> IVGGYTCQENSVPYQVSLNSGYHFCGGSLINDQWVVSAAHCYKSRIQVRLGEHNINVLEGNEQFVNAAKIIKHPNFDRKTLNNDIMLIKLSSPVKLNARVATVALPSSCAPAGTQCLISGWGNTLSSGVNEPDLLQCL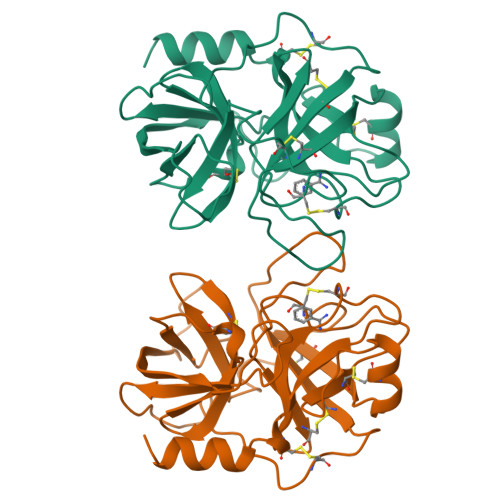DAPLLPQADCEASYPGKITDNMVCVGFLEGGKDSCQGDSGGPVVCNGELQGIVSWGYGCALPDNPGVYTKVCNYVDWIQDTIAAN>[3x]XMEMLTKFESRSSRAKGVAFHPTQPWILTSLHNGRIQLWDYRMGTLLDRFDGHDGPVRGIAFHPTQPL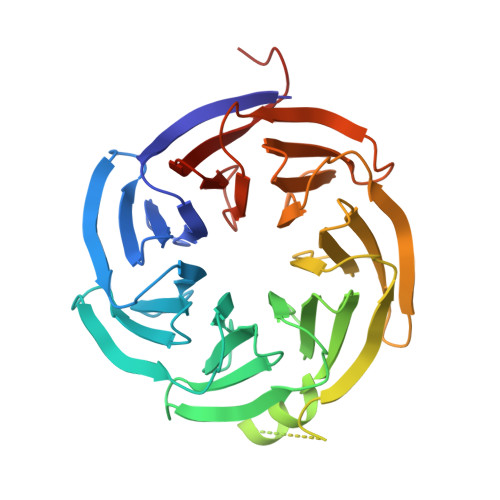FVSGGDDYKVNVWNYKSRKLLFSLCGHMDYVRVCTFHHEYPWILSCSDDQTIRIWNWQSRNCIAILTGHSHAVMCAAFHPSEDLIVSASLDQTVRVWDISGLRMKNAAPVSMSKEDQKAQAHNSKSNDKKGSTDAIVKFVLEGHDRGVNWCAFHPTLPLILSAGDDRLVKLWRMTASKAWEVDTCRGHFNNVSCCLFHPHQELILSASEDKTIRVWDLNRRTAVQTFRRDNDRFWFITVHPKLNLFAAAHDSGVMVFKLESAWSHPQFEK Isoflavonoids play important roles in plant defense and also exhibit a range of mammalian health-promoting activities. Their biosynthesis is initiated by two enzymes with unusual catalytic activities; 2-hydroxyisoflavanone synthase (2-HIS), a membrane-bound cytochrome P450 catalyzing a coupled aryl-ring migration and hydroxylation, and 2-hydroxyisoflavanone dehydratase (2-HID), a member of a large carboxylesterase family that paradoxically catalyzes dehydration of 2-hydroxyisoflavanones to isoflavone. Here we report the crystal structures of 2-HIS from Medicago truncatula and 2-HID from Pueraria lobata.

Another 2-HIS native crystal form with a P21 space group diffracted to 2.0 Å resolution, and the structure was determined using the molecular replacement method. There are two molecules in an asymmetric unit which form a dimer with extensive interactions. The heme prosthetic group was observed in the structure of 2-HIS with well-defined electron density and is located mainly between helices I and L with the I-helix on the distal side and L-helix on the proximal side, surrounded by helices C and E and the loop before helix C. Cysteine 449 acts as the 5th ligand for the iron of the heme cofactor. Remarkably, however, the location and orientation of the heme are quite different in 2-HIS compared with other P450s (e.g., human P450 2C9). The heme is moved, relative to that in human P450 2C924,25, toward helices C and E, with a distance of ~8 Å between the heme iron in the two structures, and helix C has also shifted, by ~7-8 Å. Compared with P450 2C9, the plane of the heme protoporphyrin ring in 2-HIS is tilted down ~50°. The two propionate groups also rotate ~90° towards the substrate binding pocket, a very different configuration from classical P450s, in which both propionate groups form a strong charge-charge interaction with Arg or other basic amino acids. An observed structural feature of 2-HIS is a large pocket at the edge of the heme, close to its propionate groups, and this is likely the substrate binding pocket. However, based on the present 2-HIS structure, the substrate is not able to fit on top of the heme iron, being located in a large pocket at the edge of the heme and close to its propionate groups.

>MAKKTSSKGKLPPSPKPRLPFIGHLHLLDNPLLHHTLIKLGKRYGPLYTLYFGSMPTVVASTPDLFKLFLQTHEATSFNTRFQTSAISRLTYDNSVAMVPFAPYWKFIRKLIMNDLLNATTVNKLRPLRSREILKVLKVMANSAETQQPLDVTEELLKWTNSTISTMMLGEAEEVRDIARDVLKIFGEYSVTNFIWPLNKFKFGNYDKRTEEIFNKYDPIIEKVIKKRQEIVNKRKNGEIVEGEQNVVFLDTLLEFAQDETMEIKITKEQIKGLVVDFFSAGTDSTAVSTEWTLSELINNPRVLKKAREEIDSVVGKDRLVDESDVQNLPYIKAIVKEAFRLHPPLPVVKRKCTQECEIDGYVVPEGALILFNVWAVGRDPKYWVKPLEFRPERFIENVGEGEAASIDLRGQHFTLLPFGSGRRMCPGVNLATAGMATMIASIIQCFDLQVPGQHGEILNGDYAKVSMEERPGLTVPRAHNLMCVPLARAGVADKLLSSHHHH[2x]>[5x]MYLGKVIGTVVSTSKNESLS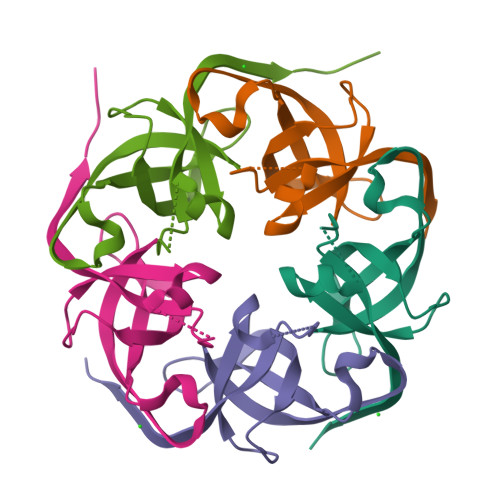GTKLLVVARLTEKLIPDGSTQVVVDTVGAGNGEIVIVSCGSSARQSTGKDHSVIDAAVVGIVDTVETVNHHHHHH> GAMGSTVGLTALKVSGETLSEPMRPGVIRFGLTPVFLSNDLEVLDELQAYLTQAVGQEVQLITQRTYQEVTALLVSGNLEAAWICGYPFMKFRDELDLVATPLWRGKPVYQSYLIVGRDRDIAGFEDCQGDIHAFSDPDSNSGYLVTKTYLAERGVSEEGFFRKSFFTYGHRNVIRAVASGLADSGSVDGYVWEVMKTTEP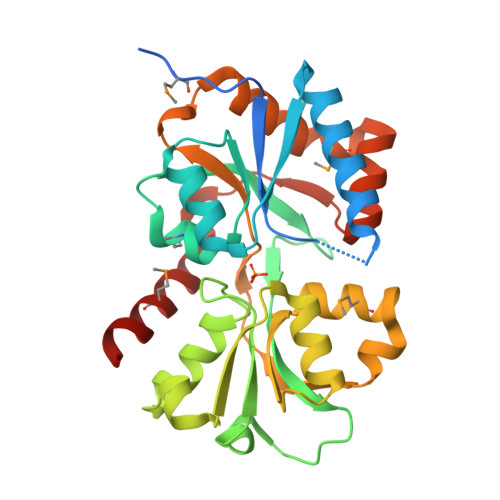ELVAKTRVLVKSGWHGFPPVAAAAGQRKSQAVARIRSALLDMNQEVLGRSVLTRLQLDGFVETTAESYDSIAANMERVRRLG> MVRNQRYPASPVQEIFLPEPVPFVQFDQTAPSPNSPPAP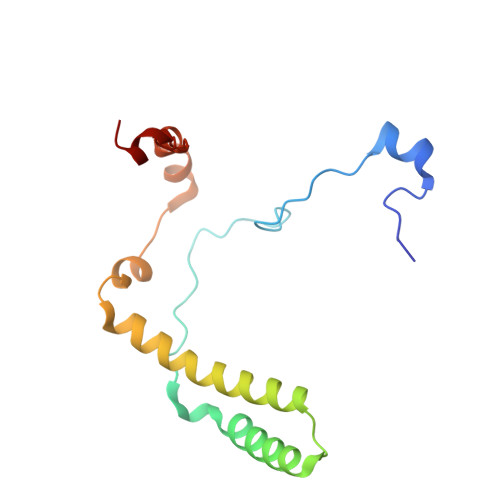LPSPSLSQCEEQKDRYRDISSMFHRGVAGAEQVREAYNSMAKCFRRVSVAEVLESDPAFRQARNFTMDLKQAEDDQRYKQLQYGRVPSILTKYHL>GSHHHHHHHHHHRSMSQTNANDLRNNEVFFISPSNNTNKVLDKISQSEVKLWNKLSGANQKWRLIYDTNKQAYKIKVMDNTSLILTWNAPLSSVSVKTDTNGDNQY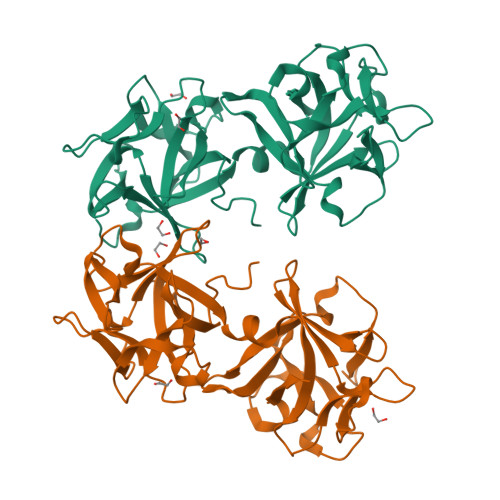WYLLQNYISRNVIIRNYMNPNLVLQYNIDDTLMVSTQTSSSNQFFKFSNCIYEALNNRNCKLQTQLNSDRFLSKNLNSQIIVLWQWFDSSRQKWIIEYNETKSAYTLKCQENNRYLTWIQNSNNYVETYQSTDSLIQYWNINYLDNDASKYILYNLQDTNRVLDVYNSQIANGTHVIVDSYHGNTNQQWIINLI[2x]>GHMASDPITTQEFSPRQNAVLDQALRLLVEGGEKALTTSGLARAANCSKESLYKWFGDRDGLLAAMITFQQSKVRTFEKAGDRVSAPQLADHLEVFAHDLLDVLAGDVSLALNRLAIGQASRDGSKLGDLLLERGRRQIDRRARGLIEAGRRSGYLRFDDAEEAYRSFYGLIVSDLHVRMLLGEAPDKDFSARAKKAVVAFLTLYGTEKVHSELGGKVAGS[2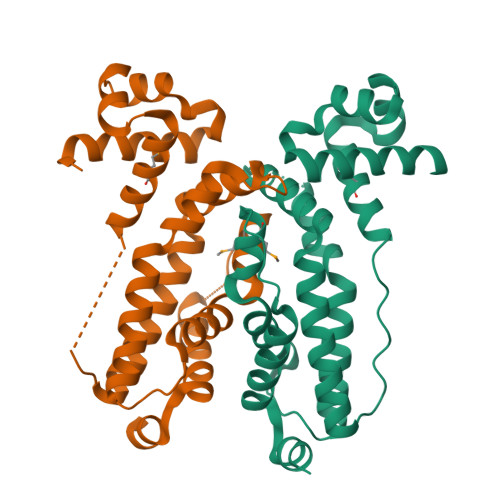x]>MPLLLLLPLLWAGALAMDKLCPLPCVCQNLSESLSTLCAHRGLLFVPPNVDRRTVELRLADNFIQALGPPDFRNMTGLVDLTLSRNAITRIGARSFGDLESLRSLHLDGNRLVELGSSSLRGPVNLQHLILSGNQLGRIAPGAFDDFLDSLEDLDVSYNNLRQVPWAGIGSMPALHTLNLDHNLIDALPPGVFAQLSQLSRLDLTSNRLATLAPDPLFSRGRDAEASPSPLVLSFSGNPLHCNCELLWLRRLARPDDLETCASPPTLAGRYFW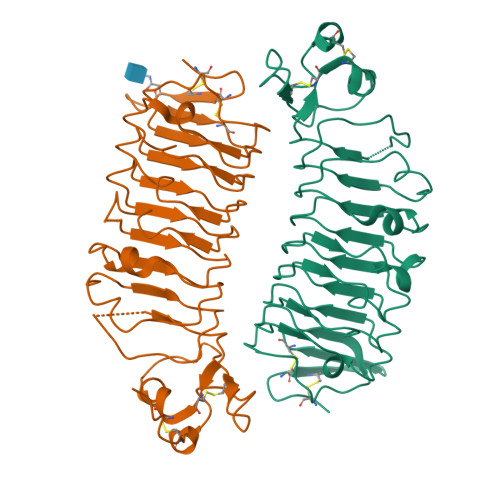AVPEGEFSCEPPLIAGTRGSLEVLFQ[4x]>[7x]GSAKDVKFGADARALMLQGVDLLADAVAVTMGPKGRTVIIEQSWGSPKVTKDGVTVAKSIDLKDKYKNIGAKLVQDVANNTNEEAGDGTTTATVLARSIAKEGFEKISKGANPVEIRRGVMLAVDAVIAELKKQSKPVTTPEEIAQVATISANGDKEIGNIISDAMKKVGRKGVITVKDGKTLNDELEIIEGMKFDRGYISPYFINTSKGQKCEFQDAYVLLSEKKISSIQSIVPALEIANA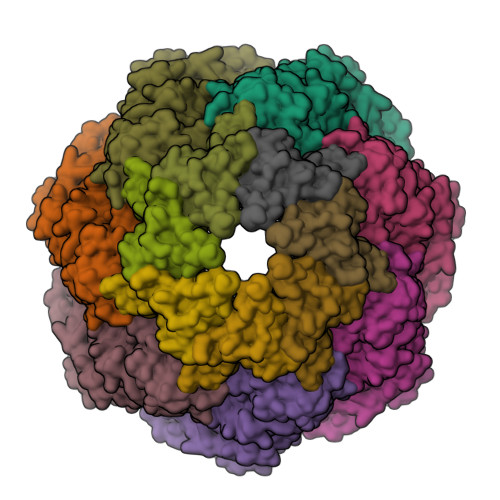HRKPLVIIAEDVDGEALSTLVLNRLKVGLQVVAVKAPGFGDNRKNQLKDMAIATGGAVFGEEGLTLNLEDVQPHDLGKVGEVIVTKDDAMLLKGKGDKAQIEKRIQEIIEQLDVTTSEYEKEKLNERLAKLSDGVAVLKVGGTSDVEVNEKKDRVTDALNATRAAVEEGIVLGGGCALLRCIPALDSLTPANEDQKIGIEIIKRTLKIPAMTIAKNAGVEGSLIVEKIMQSSSEVGYDAMAGDFVNMVEKGIIDPTKVVRTALLDAAGVASLLTTAEVVVTEIPKE;>GQAFRKFLPLFDRVLVERSAAETVTKGGIMLPEKSQGKVLQATVVAVGSGSKGKGGEIQPVSVKVGDKVLLPEYGGTKVVLDDKDYFLFRDGDILGKYVD[7x]>RKVAYLTFDDGPGKYTAELLNTLKQHDAKATFFLIGANVKEFPDLVKRENAEGHYVGMHSMTHNFAKLYKNGEYVNEMKEDQGLIANIIGKSPKLTRPPYGSMPGLNEGLRNKVVEGGFKVWDWTIDSLDWRYNKMPVDAAAAQ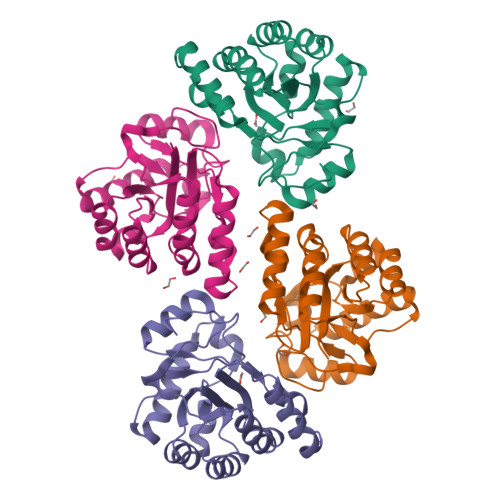IAQNVLTNATKPQEVILMHDIHPQSVAAVPAILKGLKEKGYEFEAYHEESHFPVNFWHDNRM[4x]>MANYFNTLNLRQQLAQLGKCRFMGRDEFADGASYLQGKKVVIVGCGAQGLNQGLNMRDSGLDISYALRKEAIAEKRASWRKATENGFKVGTYEELIPQADLVINLTPDKQHSDVVRTVQPLMKDGAALGYSHGFNIVEVGEQIRKDITVVMVAPKCPGTEVREEYKRGFGVPTLIAVHPENDPKGEGMAIAKAWAAATGGHRAGVLESSFVAEVKSDLMGEQTILCGMLQAGSLLCFDKLVEEGTDPAYAEKLIQFGWETITEALKQGGITLMMDRLSNPAKLRAYALSEQLKEIMAPLFQKHMDDIISGEFSSGMMADWANDDKKLLTWREETGKTAFETAPQYEGKIGEQEYFDKGVLMIAMVKAGVELAFETMVDSGIIEESAYYESLHELPL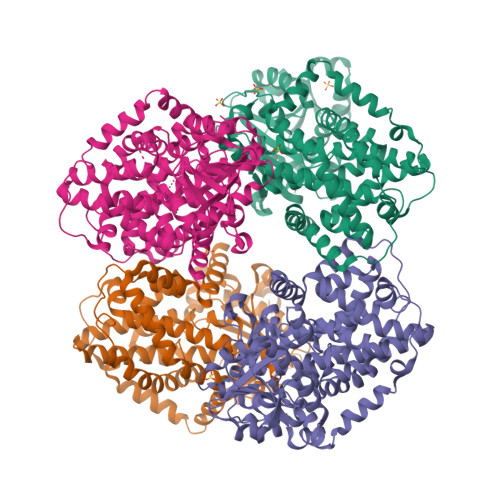IANTIARKRLYEMNVVISDTAEYGNYLFSYACVPLLKPFMAELQPGDLGKAIPEGAVDNGQLRDVNEAIRSHAIEQVGKKLRGYMTDMKRIAVAG[4x]> AGQGDGSVIELGEQTVVATAQEETKQAPGVSIITAEDIAKRPPSNDLSQIIRTMPGVNLTGNSSSGQRGNNRQIDIRGMGPENTLILVDGKPVSSRNSVRYGWRGERDSRGDTNWVPADQVERIEVIRGPAAARYGNGAAGGVVNIITKQAGAETHGNLSVYSNFPQHKAEGASERMSFGLNGPLTENLSYRVYGNIAKTDSDDWDINAGHESNRTGKQAGTLPAGREGVRNKDIDGLLSWRLTPEQTLEFEAGFSRQGNIYTGDTQNTNSNNYVKQMLGHETNRMYRETYSVTHRGEWDFGSSLAYLQYEKTRNSRINEGLAGGTEGIFDPNNAGFYTATLRDLTAHGEVNLPLHLGYEQTLTLGSEWTEQKLDDPSSNTQNTEEGGSIPGLAGKNRSSSSSARIFSLFAEDNIELMPGTMLTPGLRWDHHDIVGDNWSPSLNLSHALTERVTLKAGIARAYKAPNLYQLNPDYLLYSRGQGCYGQSTSCYLRGNDGLKAETSVNKELGIEYSHDGLVAGLTYFRNDYKNKIESGLSPVDHASGGKGDYANAAIYQWENVPKAVVEGLEGTLTLPLADGLKWSNNLTYMLQSKNKETGDVLSVTPRYTLNSMLDWQATDDLSLQATVTWYGKQKPKKYDYHGDRVTGSANDQLSPYAIAGLGGTYRLSKNLSLGAGVDNLFDKRLFRAGNAQGVVGI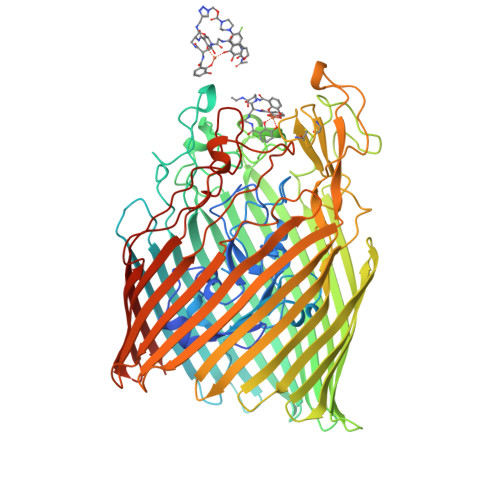DGAGAATYNEPGRTFYTSLTASF>[2x]MELRHLRYFVAVVEEQSFTKAADKLCIAQPPLSRQIQNLEEELGIQLLERGSRPVKTTPEGHFFYQYAIKLLSNVDQMVSMTKRIASVEKTIRIGFVGSLLFGLLPRIIHLYRQAHPNLRIELYEMGTKAQTEALKEGRIDAGFGRLKISDPAIKRTLLRNERLMVAVHASHPLN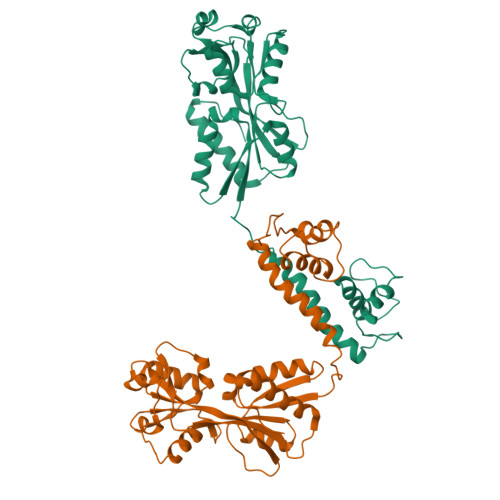QMKDKGVHLNDLIDEKILLYPSSPKPNFSTHVMNIFSDHGLEPTKINEVRKVQLALGLVAAGEGISLVPASTQSIQLFNLSYVPLLDPDAITPIYIAVRNMEESTYIYSLYETIRQIYAYEGFTEPPNWLEHHHHHH> GPGSNATQINEELYRLLEDTEILNQEITEGLLKGFEVPDAGVAIQLSKRDVVYPARILIIVLSEMWRFGLTKQSESFLAQVLTTIQKVVTQLKGNDLIPSGVFWLANVRELYSFVVFALNSILT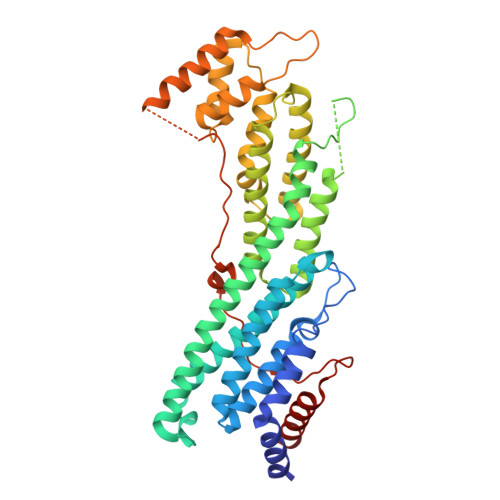EETFKNGMTDEEYKEYVSLVTELKDDFEALSYNIYNIWLKKLQKQLQKKAINAVVISESLPGFSAGETSGANTEEYTMDDILTFFNSIYWCMKSFHIENEVFHAVVTTLLNYVDAICFNELIMKRNFLSWKRGLQLNYNVTRLEEWCKTHGLTDGTECLQHLIQTAKLLQVRKYTIEDIDILRGICYSLTPAQLQKLISQYQVADYESPIPQEILRYVADIVKKEAALSSSGNDSKGHEHSSSIFITPETGPFTDPFSLIKTRKFDQVEAYIPAWLSLPSTKRIVDLVAQQVVQDGH> MKKTYRVTLTALGPIFIGGGEKLKKYEYIFDK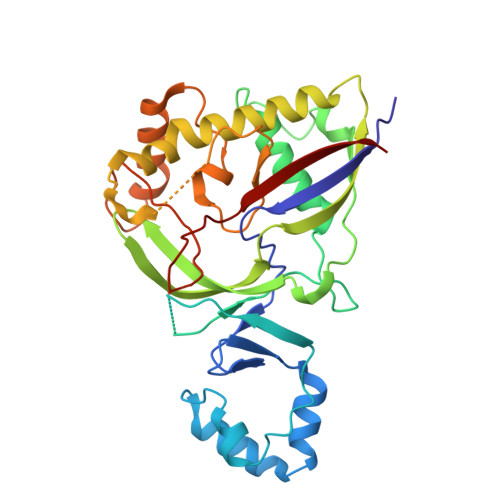QKKVAHMIDHTKFTKYLLEKNLLDDFTSRVNSHFDLYDYLVNKKGIVFMPLVKYSVPVAQFRTEVKNRFGKPISSPPMNDLNTFVKDAFGRPYIPGSSLKGALRTAILNDLKEDTKENEVFAHLQVSDSETIDLENLKVYQKVDYSKTAKPLPLYRECLKPNTEITFTVSFDDEYLTLKKIQNALHKTYQHYYIKWLKGGKVGETLIKGVYDSHADELKKNTFALDQPSQNQGEIIYIGGGAGFVSKTLHYKSKNRDQARNDSFDILKQLFRTTYSKMRSVPDNVPVALKLAVETKTFNGRVTGKHYLEMGKARIKLEEL> QTQEYTINHTGGVLGDSYVTTASNQTSPQRETAVLSFECPRKFEEINYVGQRDATRFVPRTTESITGSANDDTVVDLTANIQPVAGEEVIAEQDYPVAVAYNVTQGVEVDVVDADYAADTVTLGTNPADGDEVKVWPIMSDGDVQFRLINQFGQEEGRVYPWSTPLYRWHDFPQLKRGREINLHGSASWSENETLEILLDAPQALTWEDSDYPRG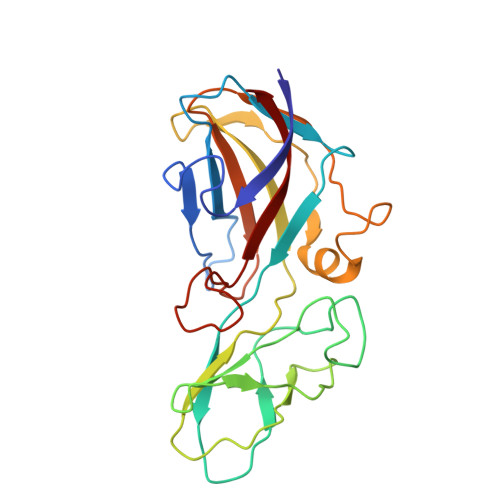QYVTTLEQDVEITL> VVVVVV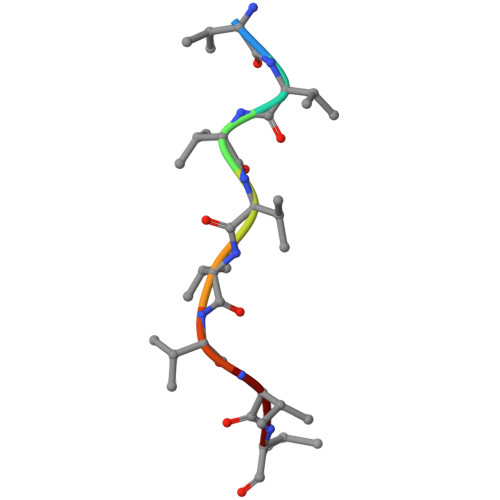VV> MGSDKIHHHHHHMSFFNKIILIGRLVRDP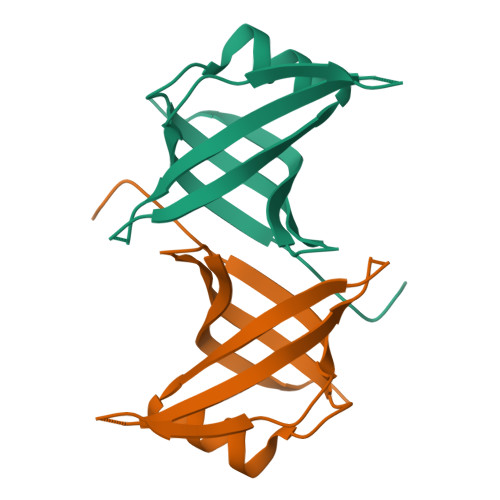EERYTLSGTPVTTFTIAVDRVPRKNAPDDAQTTDFFRIVTFGRLAEFARTYLTKGRLVLVEGEMRMRRWETPTGEKRVSPEVVANVVRFMDRKPAETVSETEEELEIPEEDFSSDTFSEDEPPF The CARMA1 signalosome, which is composed of CARMA1 (caspase recruitment domain (CARD)-containing MAGUK protein 1), BCL10 (B-cell lymphoma 10) and MALT1 (mucosa-associated lymphoid tissue lymphoma translocation protein 1), is a macromolecular complex responsible for lymphocyte activation. CARMA1 forms intracellular multi-molecular complexes with BCL10 and MALT1 that are known as CARMA1 signalosomes during lymphocytes activation and proliferation, creating a primary signaling complex for the activation of NF-κB. CARMA1 contains an N-terminal CARD (CAspase Recruitment Domain) domain followed by a coiled-coil domain and a C-terminal MAGUK domain. For assembly of the CARMA1 signalosome, CARMA1 interacts directly with BCL10 via a CARD:CARD interaction and BCL10 interacts with MALT1 via an interaction between the C-terminal Ser/Thr-rich region of BCL10 and the first Ig domain of MALT1.

In this study, we report the dimeric structure of CARMA1 CARD at a resolution of 3.2 Å. Although CARMA1 CARD has a canonical six helical-bundles structural fold similar to other CARD domains, our structure shows the first homo-dimeric structure of CARD formed by a disulfide bond and reveals a possible biologically important homo-dimeric interface and novel homo-dimerization mechanism. The high resolution structure of CARMA1 CARD showed that it forms the canonical six-helical bundle fold comprising six helices, H1 to H6, which is characteristic of the DD superfamily. There was one dimer in the asymmetric unit, referred to as chain A and chain B. A flexible loop formed by residue 64 to residue 70 was missing from our model. The electron density of that region was too weak to trace, indicating that the loop is extraordinarily flexible relative to those of other CARD domains. Interestingly, H1 of CARMA 1 CARD was bent in the middle. An electrostatic interaction between H31 from one molecule and E27 from another molecule was the only non-covalent bond detected at the interface. Interestingly, an unexpected disulfide-bond formed by C28 from each molecule was detected. CARMA1 CARD exists as dimerand further oligomer mixture in solution and was all changed to the monomeric form by the addition of DTT and by mutating C28 to Alanine, indicating that CARMA1 CARD forms a stable dimer in solution and that the dimerization is mediated by a disulfide bond.

>[2x]ALWDNVECNRHMLSRYINPAKLTPYLRQCKVIDEQDEDEVLNAPMLPSKINRAGRLLDILHTKGQRGYVVFLESLEFYYPELYKLVTGKEPTRRFSLEHHHHHH>[10x]MTTETRSLYS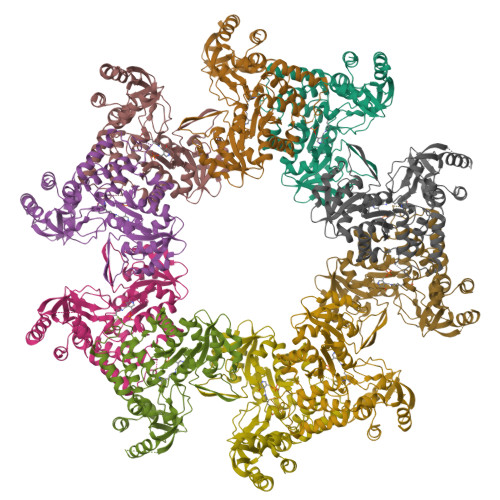QLPAIDRLLRDSSFLSLRDTYGHTRVVELLRQMLDEAREVIRGSQTLPAWCENWAQEVDARLTKEAQSALRPVINLTGTVLHTNLGRALQAEAAVEAVAQAMRSPVTLEYDLDDAGRGHRDRALAQLLCRITGAEDACIVNNNAAAVLLMLAATASGKEVVVSRGELVEIGGAFRIPDVMRQAGCTLHEVGTTNRTHANDYRQAVNENTALLMKVHTSNYSIQGFTKAIDEAELVALGKELDVPVVTDLGSGSLVDLSQYGLPKEPMPQELIAAGVSLVSFSGDKLLGGPQAGIIVGKKEMIARLQSHPLKRALRADKMTLAALEATLRLYLHPEALSEKLPTLRLLTRSAEVIQIQAQRLQAPLAAHYGAEFAVQVMPCLSQIGSGSLPVDRLPSAALTFTPHDGRGSHLESLAARWRELPVPVIGRIYDGRLWLDLRCLEDEQRFLEMLLK>MNGVLIPHTPIAVDFWSLRRAGTARLFFLSHMHSDHTVGLSSTWARPLYCSPITAHLLHRHLQVSKQWIQALEVGESHVLPLDEIGQETMTVTLLDANHCPGSVMFLFEGYFGTILYTGDFRYTPSMLKEPALTLGKQIHTLYLDNTNCNPALVLPSRQEAAHQIVQLIRKHPQHNIKIGLYSLGKESLLEQLALEFQTWVVLSPRRLELVQLLGLADVFTVEEKAGRIHAVDHMEICHSNMLRWNQTHPTIAILPTSRKIHSSHPDIHVIPYSDHSSYSELRAFVAALKPCQVVPIVSRRPCGGFQDSLSPRISVPLIPDSVQQYMSSSSRKPSAENLYFQ[2x]

Human SNM1B (SNM1B, Apollo, or DCLRE1B) is a 5′-to-3′ exonuclease, which was first identified as one of three vertebrate orthologues of the yeast DNA repair nuclease, PSO2 (4). SNM1B is a member of the metallo-β-lactamase (MBL) structural superfamily, of which the β-CASP (CPSF, Artemis, SNM1, PSO2) nucleic acid processing nucleases are a subfamily. All MBL type enzymes possess a characteristic α/β/β/α MBL core fold that provides a scaffold that supports the active site, which coordinates the metal ions essential for catalysis. The SNM1B sequence comprises 532 amino acids, wherein the N-terminal region (amino acids 1–332) contains the catalytic (MBL and β-CASP) domains, and the C-terminal region the protein-protein interaction regions, including the well-characterised TRF2 binding domain (amino acids 498–509).

To gain insight into the SNM1B reaction mechanism, we obtained crystal structures with relevant active site binding ligands, solving a co-crystal structure of a C-terminally truncated form of SNM1B (amino acids 1–335) with two 2′-deoxy-5′-adenosine monophosphate (AMP) molecules at the active site (denoted SNM1B (nucleotide form)). The two 2′-deoxy-5′-AMP (AMP_1 and AMP_2) molecules are bound in the active site and are arranged in a position consistent with that predicted for the terminal nucleotide products from hydrolysis of a ssDNA substrate. The first nucleotide (AMP_1) is bound in a well-defined pocket formed in the cleft between the MBL and β-CASP domains. The 5′-phosphate group is located at the base of this pocket, and makes extensive protein interactions, including seven hydrogen bonds via the main chain amides of S258 and D275, the sidechain hydroxyls of Y182, T257, S258 and S274, and a single positively charged sidechain of K186. Whilst the ribose sugar does not appear to form any direct protein interactions, binding of the adenine base is stabilized by stacking with the guanidium sidechains of R301 and R259, involving cation-π type interactions. The 5′-phosphate group of AMP_2 is located where the phosphodiester bond is predicted to be, prior to substrate cleavage. Two 5′-phosphate oxygen atoms (O1 and O3) of AMP_2 coordinate to one of the metal ions, whilst the third phosphate oxygen is positioned to form a hydrogen bond / electrostatic interaction with NE2 of imidazole sidechain of H276 (motif B; β-CASP domain). Although we cannot be sure of the Fe/Ni distribution between the two sites, analysis of related metal ion binding sites led us to model a Ni2+ at the M1 site (according to canonical MBL nomenclature), coordinated by H31 and H33 (motif 2; MBL domain), H99 (motif 3; MBL domain), D120 (motif 4; MBL domain), and a water molecule. The second metal ion (M2 site) was modelled as an Fe; it is coordinated in an octahedral arrangement by D35A and H36A (motif 2; MBL domain), D120 (motif 4; MBL domain), an oxygen (O1) of the 5′-phosphate group of AMP_2, and two water molecules.Factor XI (FXI) has an important role in thrombin generation in the amplification phase of the coagulation process. Inhibition of activated FXI (FXIa) should decrease thrombin generation in the amplification phase, but not in the initiation phase, and thus yield an antithrombotic and profibrinolytic effect with minimal risk of bleeding (see reviews). To improve crystallisability, the quadruple mutant (Ser75Ala, Lys78Ala, Thr97Ala and Cys123Ser), first reported by Jin et al., was generated. The mutated residues in this construct (FXIa CD) are located at least 16 Å from the catalytic residue Ser195 and the alterations are therefore not anticipated to impact ligand binding in the active site.

Several of the fragment hit compounds were only weakly basic, such as aminopyridines and aminoquinolines, and neutral compounds, such as chloroquinolinones and the known p-chlorophenyltetrazoles, were also identified. Two prioritized fragment hits, 6-chloro-3,4-dihydro-1H-quinolin-2-one and 4-methylquinolin-6-amine are shown in Fig. 5. To our knowledge, 5 is a novel serine protease P1 structure, and 6 is here described for the first time to bind FXIa. The crystal structures of compounds 5 and 6 in complex with FXIa were solved to 2.0 and 1.7 Å resolution, respectively, and the fragments could be unambiguously placed in the electron density maps. The two fragments display distinct binding modes as depicted in Fig. 5. Fragment 5 displayed a FXIa IC50 of 140 μM. The chloro atom is directed almost perpendicular to the aromatic ring of Tyr228 and is located at a distance of 3.8 Å to the closest carbon atom of the phenyl ring. This chloro atom replaces a highly conserved water molecule and its position is similar to the chloro atom in chloro-phenyl containing P1s of FXIa, thrombin and FXa inhibitor. The chloroquinolinone compound 5 picks up an additional interaction with FXIa, i.e. the quinolinone NH group forms a 2.7 Å hydrogen bond with the backbone carbonyl of Gly218. Notably, the chloroquinolinone is slightly more potent than benzamidine, compound 7, despite the fact that the former is neutral and does not form polar interactions with Asp189. This suggests that the chloroquinolinone P1 is a promising FXIa fragment inhibitor, with potential to be expanded and developed into an orally active drug.

> IVGGTASVRGEWPWQVTLHTTSPTQRHLCGGSIIGNQWILTAAHCFYGVESPKILRVYSGILNQAEIAEDTSFFGVQEIIIHDQYKMAESGYDIALLKLETTVNYADSQRPISLPSKGDRNVIYTDCWVTGWGYRKLRDKIQNTLQKAKIPLVTNEECQKRYRGHKITHKMICAGYREGGKDACKGDSGGPLSCKHNEVWHLVGITSWGEGCAQRERPGVYTNVVEYVDWILEKTQAV>[4x]AMGKKVLIVYAHQEPKSFNGSLKNVAVDELSRQGCTVTVSDLYAMNFEPRATDKDITGTLSNPEVFNYGV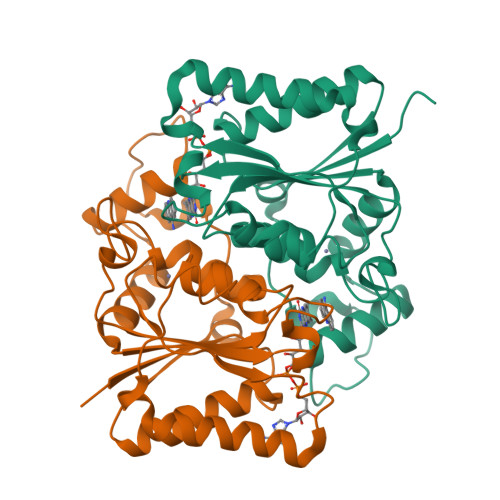ETHEAYKQRSLASDITDEQKKVREADLVIFQFPLYWFSVPAILKGWMDRVLCQGFAFDIPGFYDSGLLQGKLALLSVTTGGTAEMYTKTGVNGDSRYFLWPLQHGTLHFCGFKVLAPQISFAPEIASEEERKGMVAAWSQRLQTIWKEEPIPCTAHWHFG>[2x]GSHMSKPVKSKTTGKNIGYGKVILFGEHFVVHGAEAIVAGISEYTECRLEINPGVPGLQVDDQRPAIPGYIAQKRDEQIK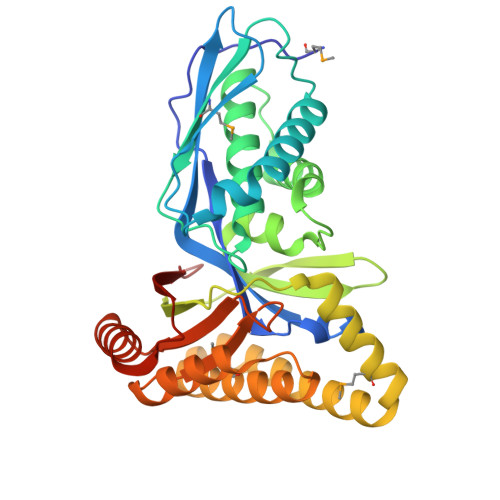AHQLVLDHLKVDLSGDGLKMFIGGPLVPSSGIGASASDVVAFSRALSELYQLNLTDEEVNLSAFVGEGGYHGTPSGADNTAATYGGLILYRRQNGKSVFKPIAFQQRLYLVVVGTGINASTAKVVNDVHKMKQQQPVQFKRLYDNYTHIVSQAREALQKGDLQRLGQLMNANHDLCRQIDVSCRELESIVQTCRTYGALGAKLSGTGRGGIAVALAASSDQRDAIVKGLKAKCPEAKFIWRYTVQPSAASNL Cry78Aa is a novel protein identified from the Bt C9F1 strain that effectively kills rice planthoppers, with median lethal concentration (LC50) values against Laodelphax striatellus and Nilaparvata lugens of 6.89 and 15.78 μg ml−1, respectively. Here, we report the crystal structure of Cry78Aa, which consists of two domains: a C-terminal β-pore forming domain belonging to the aerolysin family and an N-terminal trefoil domain resembling the S-type ricin B lectin. We also found that Cry78Aa binds carbohydrates such as galactose derivatives and is essential for insecticidal activity against Laodelphax striatellus. Bioassays showed that the NTD or CTD of Cry78Aa alone has no toxicity against planthopper nymphs, indicating that its insecticidal activity is dependent on the cooperation of both domains.

Here, we resolved the crystal structure of Cry78Aa13-359, which approximately resembles full-length Cry78Aa. Consequently, the structure of Cry78Aa13-359 was resolved by combining SAD with molecular replacement using Cry78Aa155-359 as a model. The final structure of Cry78Aa13-359 was refined to 2.9 Å resolution with Rwork and Rfree values of 0.279 and 0.282, respectively. Cry78Aa13-359 exists as an X-shaped tetramer in the crystal structure and the four molecules are nearly identical to each other. Mol A and Mol B are arranged in one plane, and Mol C and Mol D symmetrically protrude from the plane by ~15 degrees. Taking one protomer (Mol A) as an example, monomeric Cry78Aa13-359 exhibits a rigid rod-like shape and comprises two domains, the NTD and the CTD. The NTD of Cry78Aa13-359 has a typical trefoil shape which is usually composed of three sets of β-sheets and is also known as the trefoil domain. The CTD of Cry78Aa13-359 is mainly composed of several long parallel β-sheets and three α-helices, and is regarded as a β-pore-forming domain. The NTD of Cry78Aa13-359 glues four protein molecules together.

>[4x]AHMNEIDNGIKALDPFNFYRIRTFCGKMLDVVGQSTSDNAMVVQYSINNKPNQNFLVFTLDDGYSIIAAENSGKVLDISEDFFFKGMLIQYHFANSDNQKFLISNNGTIAVKRSGKVFDIPGASTSNDAPVIAYNFNNAANQKFTFERVKTFQVPSPSIGTLPPAPDFKNDINEQLPDKTNPVITHFSTIPYIMANDATFNSHQQIQYSPYYKLVRIQYWEKVTQRILGPRDDYEYNKTKGISKTDQVSMTETVSMSVGADFGFMFKGFSASLSAQITKELSVTKSTSTTEMTEETYKEKYTNPFNYELARAQYMLVNEFYVTRMDGTRITANWTLRDNTQTVTRIFPKS>APKRKSGVSKCETKCTKACPRPAPVPKLLIKGGMEVLDLVTGPDSVTEIEAFLNPRMGQPPTPESLTEGGQYYGWSRGINLATSDTEDSPENNTLPTWSMAKLQLPMLNEDLTCDTLQMWEAVSVKTEVVGSGSLLDVHGFNKPTDTVNTKGISTPVEGSQYHVFAVGGEPLDLQGLVTDARTKYKEEGVVTIKTITKKDMVNKDQVLNPISKAKLDKDGMYPVEIWHPDPAKNENTRYFGNYTGGTTTPPVLQFTNTLTTVLLDENGVGPLCKGEGLYLSCVDIMGWRVTRNYDVHHWRGLPRYFKITLRKRWVKNPYPMASLI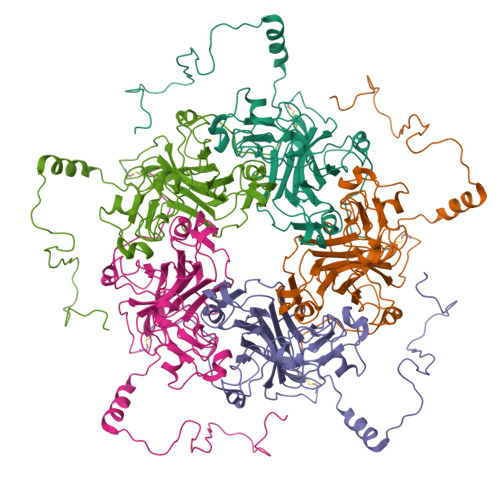SSLFNNMLPQVQGQPMEGENTQVEEVRVYDGTEPVPGDPDMTRYVDRFGKTKTVFPGN[5x]> GSHMSYQKVPNSHKEFTKFCYEVYNEIKISDKEFKEKRAALDTLRLCLKRISPDAELVAFGSLESGLALKNSDMDLCVLMDSRVQSDTIALQFYEELIAEGFEGKFLQRARIPIIKLTSDTKNGFGASFQCDIGFNNRLAIHNTLLLSSYTKLDARLKPMVLLVKHWAKRKQINSPYFGTLSSYGYVLMVLYYLIHVIKPPVFPNLLLSPLKQEKIVDGFDVGFDDKLEDIPPSQNYSSLG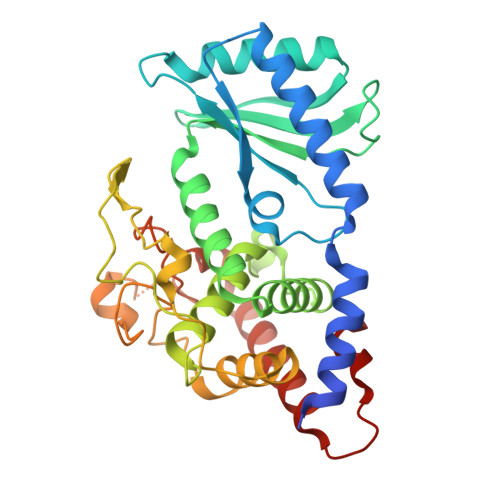SLLHGFFRFYAYKFEPREKVVTFRRPDGYLTKQEKGWTSATEHTGSADQIIKDRYILAIEDPFEISHNVGRTVSSSGLYRIRGEFMAASRLLNSRSYPIPYDSLFEEA>GSHMEGLVVAAGGDVSLHNFSARLWEQLVHFHVMRLTDSLFLWVGATPHLRNLAVAMSSRYDSIPVSTSLLGDTSDTTSTGLAQRLARKTNKQVFVSYN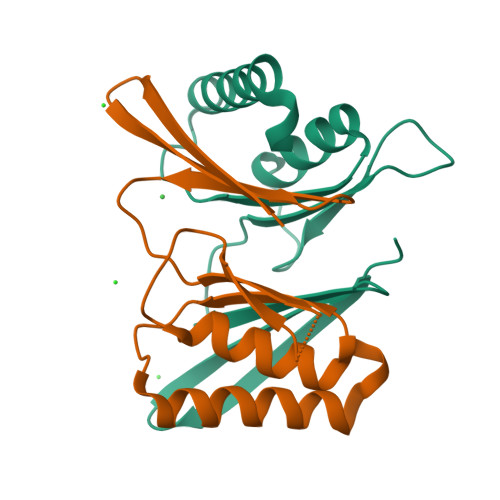LQNTDSNFALLVENRIKEEMEAFPEKF[4x]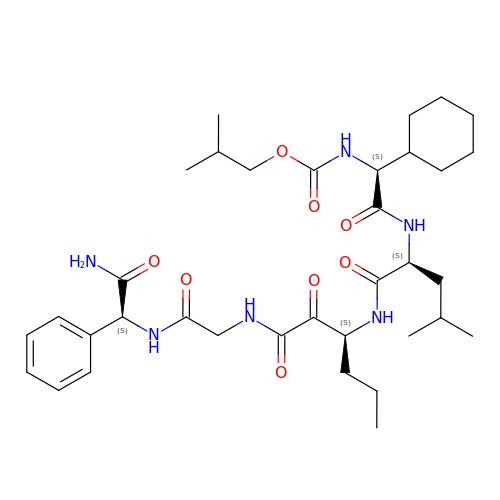({1-[1-CARBAMOYL-PHENYL-METHYL)-CARBAMOYL]-METHYL}-AMINOOXALYL)-BUTYLCARBAMOYL)-3-METHYL-BUTYLCARBAMOYL)-CYCLOHEXYL-METHYL)-CARBAMIC ACID ISOBUTYL ESTER | C35 H54 N6 O8 | CSOCTFLGSKTNFD-DZXSPZCNSA-N3-AMINOPROPANE | C3 H9 N | 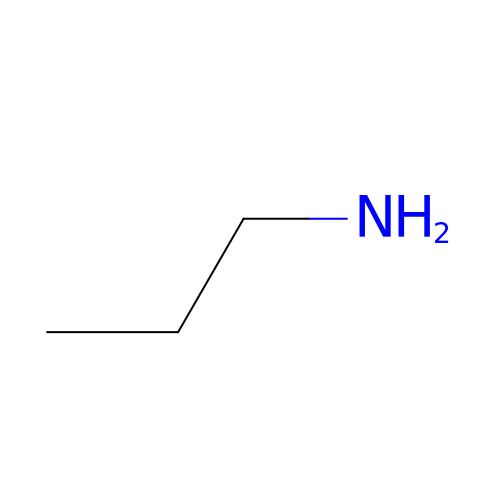WGYKZJWCGVVSQN-UHFFFAOYSA-N>[3x]ATAAEIAALPRQKVELVDPPFVHAHSQVAEGGPKVVEFTMVIEEKKIVIDDAGTEVHAMAFNGTVPGPLMVVHQDDYLELTLINPET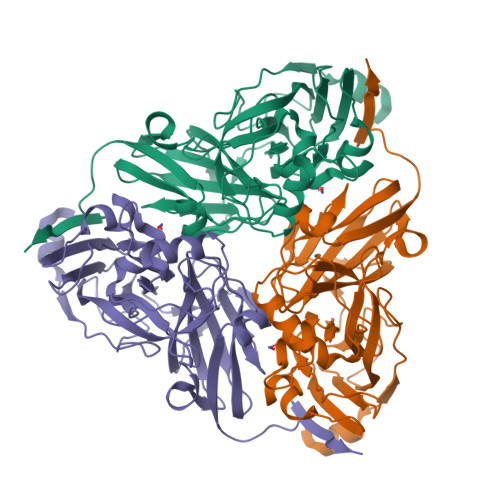NTLMHNIDFHAATGALGGGGLTEINPGEKTILRFKATKPGVFVYHCAPPGMVPWHVVSGMNGAIMVLPREGLHDGKGKALTYDKIYYVGEQDFYVPRDENGKYKKYEAPGDAYEDTVKVMRTLTPTHVVFNGAVGALTGDKAMTAAVGEKVLIVHSQANRDTRPHLVGGHGDYVWATGKFNTPPDVDQETWFIPGGAAGAAFYTFQQPGIYAYVNHNLIEAFELGAAAHFKVTGEWNDDLMTSVLAPSGTIEGR>SNAMNDIVASTQLPNTIKTITNDLRKLGLKKGMTVIVHSSLSSIGWISGGAVAVVEALMEVITEEGTIIMPTQSSDLSDPKHWSRPPVPEEWWQIIR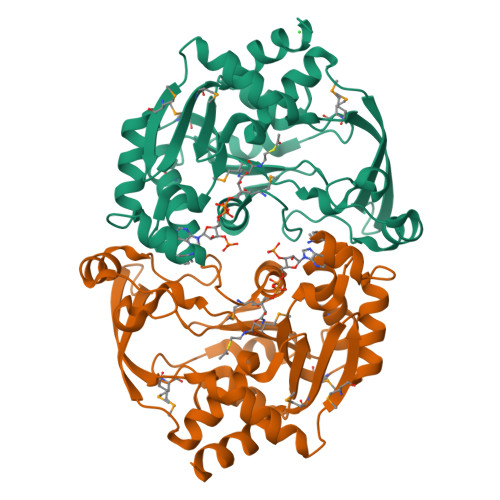DNVPAFEPHITPTRAMGKVVECFRTYPNVVRSNHPLGSFAAWGRHAEEITVNQSLSMSLGEESPLRKIYDLDGYILLIGVGYDSNTSVGLSEVRSGACELIKVGAPIIENGERVWKEFVDMDYDSDKFVEIGVEFEQKGTVTMGKIGNAKCRLMKQRDIVDFGTEWFRKKN[2x]> KVEQAVETEPEPELRQQTEWQSGQRWELALGRFWDYLRWVQTLSEQVQEELLSSQVTQELRALMDETMKELKAYKSELEEQLTPVAEETRARLSKELQAAQARLGADMEDVCGRLVQYRGEVQAMLGQSTEELRVRLASHLRKLRERLLRDADDLQKRLA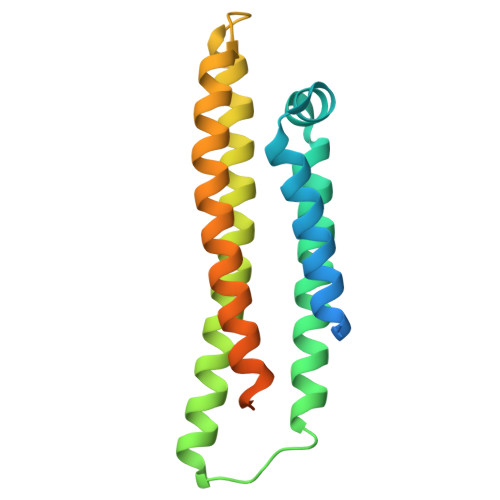VYQAGAREGAERGLSAIRERLGPLVEQGRVR>[2x]GPRFLKVKNWETDVVLTDTLHLKSTLETGCTEHICMGSIMLPSQHTRKPEDVRTKDQLFPLAKEFLDQYYSSIKRFGSKAHMDRLEEVNKEIESTSTYQLKDT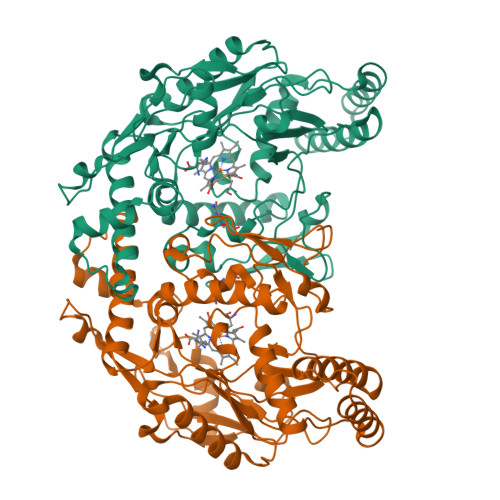ELIYGAKHAWRNASRCVGRIQWSKLQVFDARDCTTAHGMFNYICNHVKYATNKGNLRSAITIFPQRTDGKHDFRVWNSQLIRYAGYKQPDGSTLGDPANVQFTEICIQQGWKAPRGRFDVLPLLLQANGNDPELFQIPPELVLEVPIRHPKFDWFKDLGLKWYGLPAVSNMLLEIGGLEFSACPFSGWYMGTEIGVRDYCDNSRYNILEEVAKKMDLDMRKTSSLWKDQALVEINIAVLYSFQSDKVTIVDHHSATESFIKHMENEYRCRGGCPADWVWIVPPMSGSITPVFHQEMLNYRLTPSFEYQPDPWNTHVW>[2x]MTSFQEVPLQTSNFAHVIFQNVAKSYLPNAHLECHYTLTPYIHPHPKDWVGIFKVGWSTARDY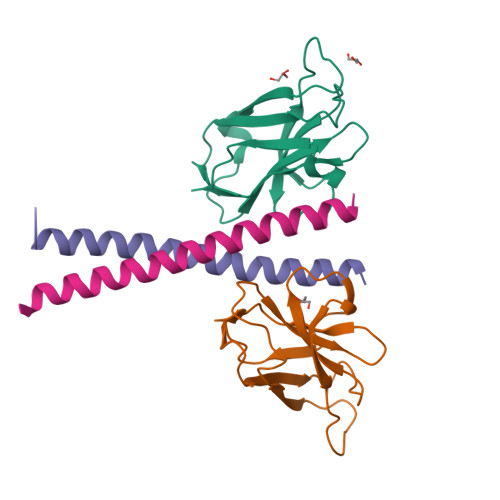YTFLWSPMPEHYVEGSTVNCVLAFQGYYLPNDDGEFYQFCYVTHKGEIRGASTPFQFR;>ESVASHFALVTAYEDIKKRLKDSEKENSLLKKRIRFLEEKLIA[2x]> VKLSHVEKDFIAFYSTTPHHLSYRDKTGGSYFITRLISCFRKHACSCHLFDIFLKVQQS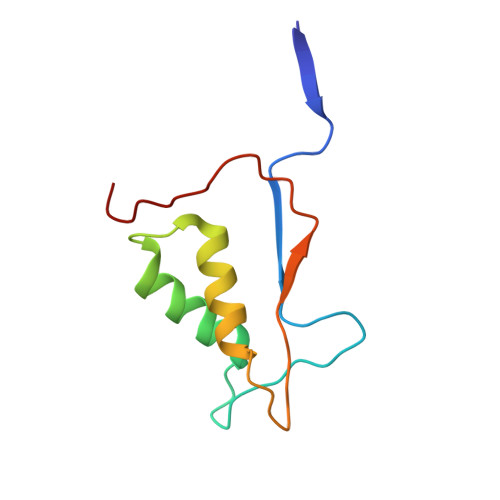FEKASIHSQMPTIDRATLTRYFYLFPGN> TTGVYVKM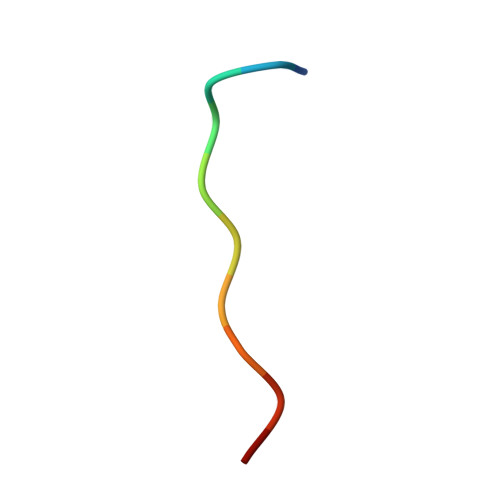PPT>[2x]GHMAIAPNTRVLVAGYGLPAEFCVTTLIGMGVEIDKIAVATHREDNRNCGLHSMLRLRNIQF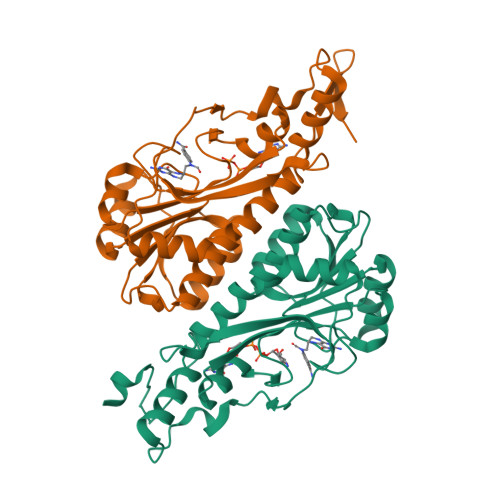TTAAANSEEFYEFGANFAPDMIISMHYRSLIPGRFLKLAKKGSVNLHPSLLPAYRGTNSVAWVIINGESETGFSYHRMDENADTGAILLQERISVEETDTAFSLFHRQIARAMLRLEEVILKLDQGDPGFAQLGEASYYARELPFGGVIDPRWSEVQIDRFIRAMFFPPFPPAVLKIDGKVYYVPSIDIYRSLMRGIPS> NQSVVVDFLLPTGVYLNFPVSRNANLSTIKQLLWHRAQYEPLFHMLSGPEAYVFTCINQTAEQQELEDEQRRLCDVQPFLPVLRLVAREGDRVKKLINSQISLLIGKGLHEFDSLCDPEVNDFRAKMCQFCEEAAARRQQLGWEAWLQYSFPLQLEPSAQTWGPGTLRLPNRALLVNVKFEGSEESFTFQVSTKDVPLALMACALRKKATVFRQPLVEQPEDYTLQVNGRHEYLYGSYPLCQFQYICSCLHSGLTPHLTMVHSSSILAMRDEQSNPAPQVQKPRAKPPPIPAKKPSSVSLWSLEQPFRIELIQGSKVNADERMKLVVQAGLFHGNEMLCKTVSSSEVSVCSEPVWKQRLEFDINICDLPRMARLCFALYAVIEKAKKARSTKKKSKKADCPIAWANLMLFDYKDQLKTGERCLYMWPSVPDEKGELLNPTGTVRSNPNTDSAAALLICLPEVAPHPVYYPALEKILELG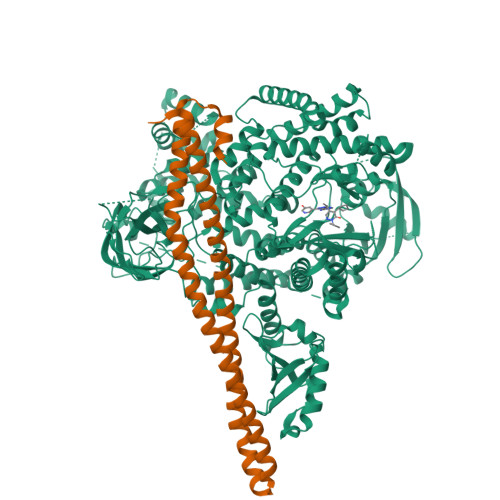RHSECVHVTEEEQLQLREILERRGSGELYEHEKDLVWKLRHEVQEHFPEALARLLLVTKWNKHEDVAQMLYLLCSWPELPVLSALELLDFSFPDCHVGSFAIKSLRKLTDDELFQYLLQLVQVLKYESYLDCELTKFLLDRALANRKIGHFLFWHLRSEMHVPSVALRFGLILEAYCRGSTHHMKVLMKQGEALSKLKALNDFVKLSSQKTPKPQTKELMHLCMRQEAYLEALSHLQSPLDPSTLLAEVCVEQCTFMDSKMKPLWIMYSNEEAGSGGSVGIIFKNGDDLRQDMLTLQMIQLMDVLWKQEGLDLRMTPYGCLPTGDRTGLIEVVLRSDTIANIQLNKSNMAATAAFNKDALLNWLKSKNPGEALDRAIEEFTLSCAGYCVATYVLGIGDRHSDNIMIRESGQLFHIDFGHFLGNFKTKFGINRERVPFILTYDFVHVIQQGKTNNSEKFERFRGYCERAYTILRRHGLLFLHLFALMRAAGLPELSCSKDIQYLKDSLALGKTEEEALKHFRVKFNEALRESWKTKVNWL;> YQQDQVVKEDNIEAVGKKLHEYNTQFQEKSREYDRLYEDYTRTSQEIQMKRTAIEAFNETIKIFEEQCQTQERYSKEYIEKFKREGNETEIQRIMHNYEKLKSRISEIVDSRRRLEEDLKKQAAEYREIDKRMNSIKPDLIQLRKTRDQYLMWLTQKGVRQKKLNEWLG> SNAMSDTLRPYKNLFPGIGQRVMIDTSSVVIGDVRLADDVGIWPLVVIRGDVNYVAIGARTNIQDGSVLHVT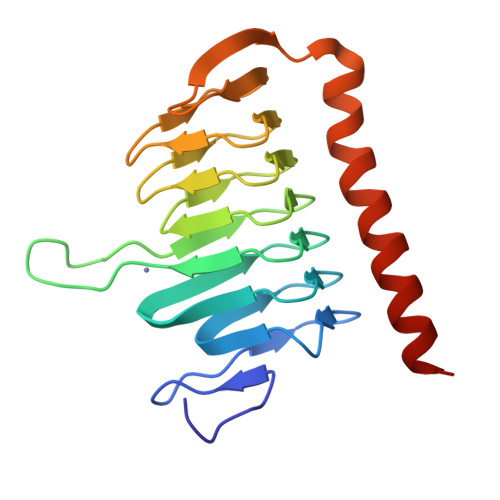HKSSSNPHGNPLIIGEDVTVGHKVMLHGCTIGNRVLVGMGSIVLDGAIIEDDVMIGAGSLVPQHKRLESGYLYLGSPVKQIRPLSDAERSGLQYSANNYVKWKDDYLSQDNHIQP>MNLNIVPLFEKTLSASDAGRIGRLVLPKACAEAYFPPISQSEGIPLKIQDVRGREWTFQFRYWPNNNSRMYVLEGVTPCIQSM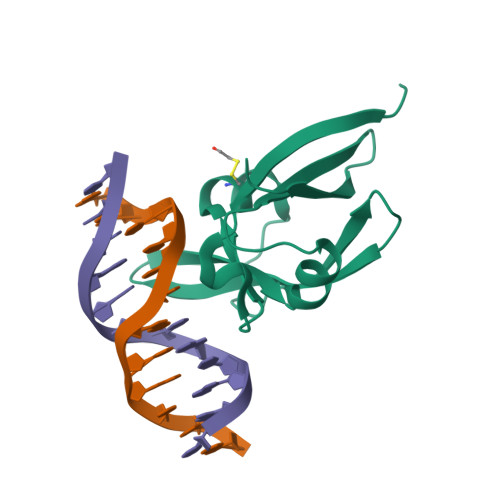MLQAGDTVTFSRVDPGGKLIMGSRKAANGHHHHHHG[2x]> SVIEKLRKLE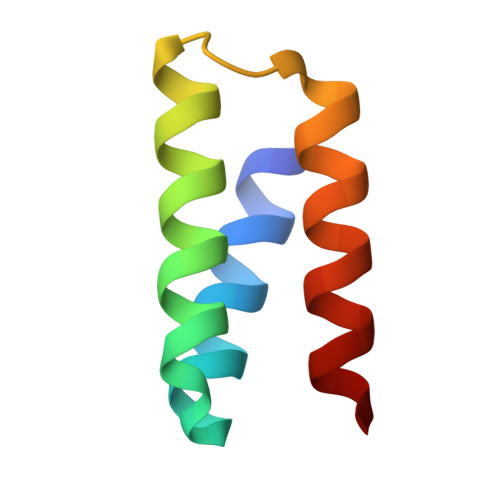KQARKQGDEVLVMLARMVLEYLEKGWVSEEDADESADRIEEVLKK>[8x]AETVSFNFNSFSEGNPAINFQGDVTVLSNGNIQLTNLNKVNSVGRVLYAMPVRIWSSATGNVASFLTSFSFEMKDIKDYDPA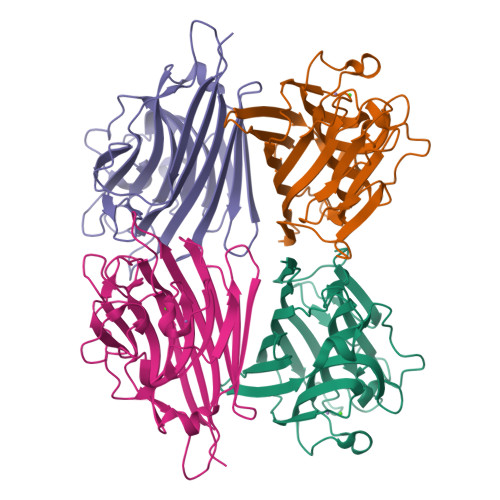DGIIFFIAPEDTQIPAGSIGGGTLGVSDTKGAGHFVGVEFDTYSNSEYNDPPTDHVGIDVNSVDSVKTVPWNSVSGAVVKVTVIYDSSTKTLSVAVTNDNGDITTIAQVVDLKAKLPERVKFGFSASGSLGGRQIHLIRSWSFTSTLITT>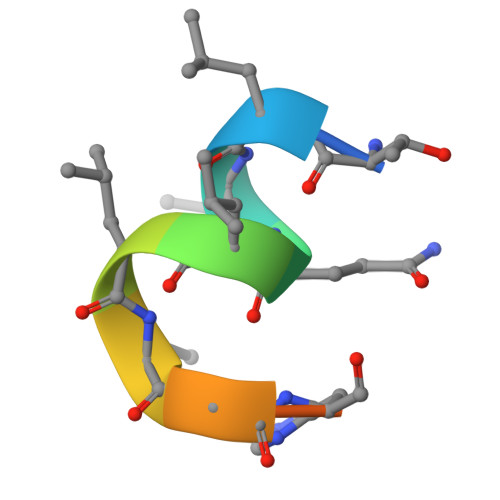 TLLQLLLGHKNE>MIRFLEKYVMPVAGKVAEQRHLLAIRDGLVLTMPFLIIGSIFLIISTLPIPGYSEFMASLFGKNWNVALGYPVSATFNIMALIAVFGIAYRLGEYYKVDALASGALSLVTFLLATPFQVAYIMPGTKESILVDGVIPAALMGSQGLFVAMIIAIISTEIYRFLVQKKMIIKMPETVPPAVTRSFAALIPGFIVVTVVWIIRLIFEHTTFGSIHNVVGKLLQEPLSILGASLWGAVIAVILVHVLWACGIHGATIVGGVMSPIWLSLMDQNRIAFQAGQDVPNTITAQFFDLWIYMGGSGATLALVVGMLLFARSQQLKSLGRLSIAPGIFNINEMVTFGMPIVMNPLLLIPFIVVPVVLT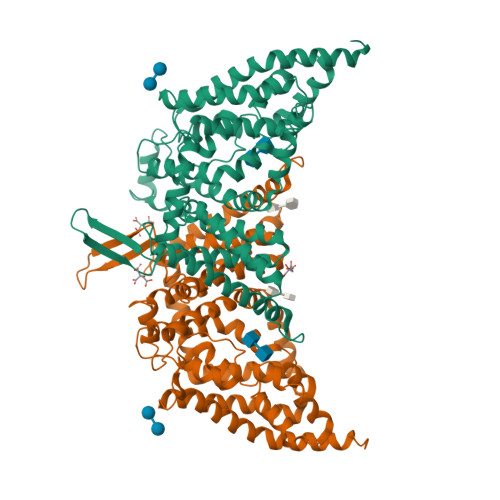IVSYFAMEWGLVARPSGAAVTWTTPILFSGYLGSGGKISGVILQLVNFALAFVIYLPFLKIWDKQKIAEEKGEAAAENLYFQ[4x]>[2x]MKTPEDCTGLADIREAIDRIDLDIVQALGRRMDYVKAASRFKASEAAIPAPERV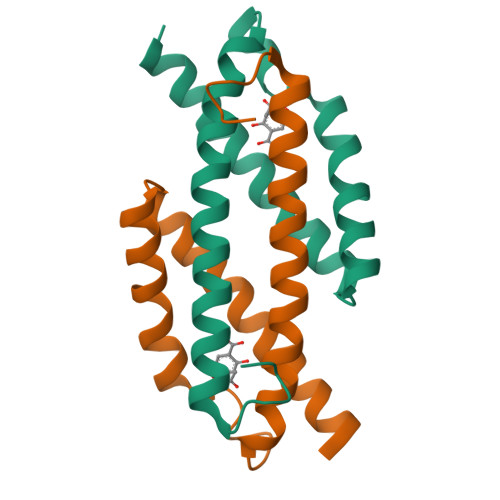AAMLPERARWAEENGLDAPFVEGLFAQIIHWYIAEQIKYWRQTRGAA>[12x]MSELFSERIPPQSIEAEQAVLGAVFLDPAALVPASEILIPEDFYRAAHQKIFHAMLRVADRGEPVDLVTVTAELAASEQLEEIGGVSYLSELADAVPTAANVEYYARIVEEKSVLRRLIRTATSIAQDGYTREDEIDVLLDEADRKIMEVSQRKHSGAFKNIKDILVQTYDNIEMLHNRDGEITGIPTGFTELDRMTSGFQRSDL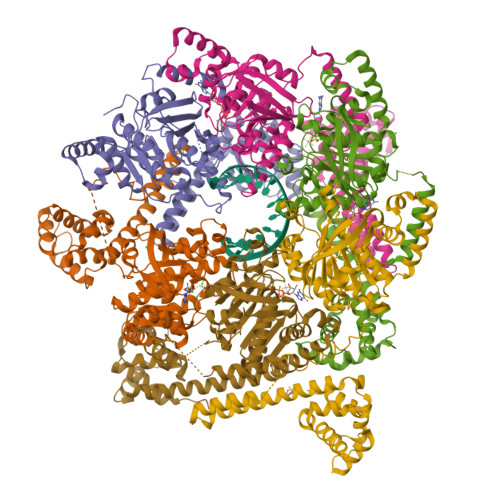IIVAARPSVGKTAFALNIAQNVATKTNENVAIFSLEMSAQQLVMRMLCAEGNINAQNLRTGKLTPEDWGKLTMAMGSLSNAGIYIDDTPSIRVSDIRAKCRRLKQESGLGMIVIDYLQLIQGSGRSKENRQQEVSEISRSLKALARELEVPVIALSQLSRSVEQRQDKRPMMSDIRESGSIEQDADIVAFLYRDDYYNKDSENKNIIEIIIAKQRNGPVGTVQLAFIKEYNKFVNLERRFDEAQIPPGA> KDLLKGLDQEQANEVIAVLQMHNIEANKIDSGKLGYSITVAEPDFTAAVYWIKTYQLPPRPRVEIAQMFPADSLVSSPRAEKA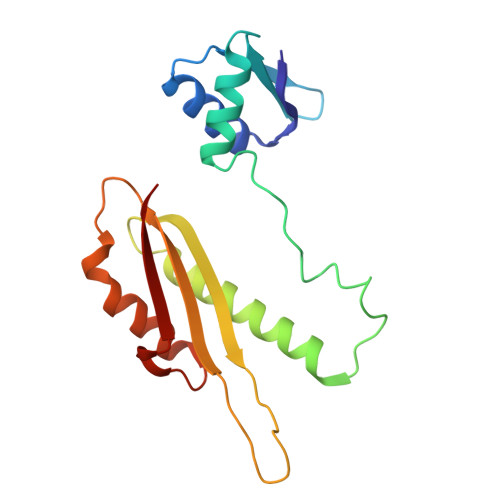RLYSAIEQRLEQSLQTMEGVLSARVHISYDIDAGENGRPPKPVHLSALAVYERGSPLAHQISDIKRFLKNSFADVDYDNISVVLSER>[2x]MNITKTLCLCAALSGAAGVQAMENREFVTQQDNTRVNNYQTNRPEAS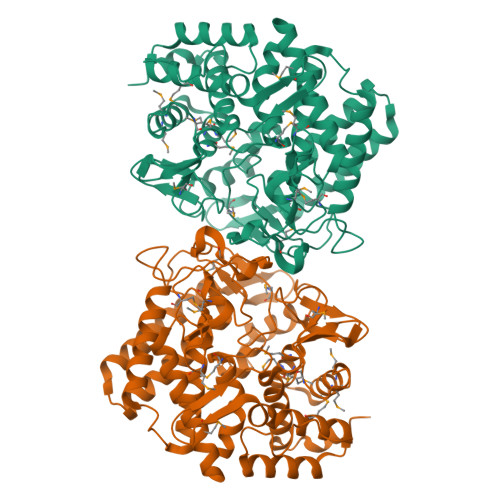KRLFVSQEVERQIDHIKQLLTNAKLAWMFENCFPNTLDTTVHFDGKEDTFVYTGDIHAMWLRDSGAQVWPYVQLANKDPELKKMLAGVINRQFKCINIDPYANAFNMNSEGGEWMSDLTDMKPELHERKWEIDSLCYPIRLAYHYWKTTGDASVFSDEWLQAIANVLKTFKEQQRKDDAKGPYRFQRKTERALDTMTNDGWGNPVKPVGLIASAFRPSDDATTFQFLVPSNFFAVTSLRKAAEILNTVNRKPALAKECTALADEVEKALKKYAVCNHPKYGKIYAFEVDGFGNQLLMDDANVPSLIALPYLGDVKVTDPIYQNTRKFVWSEDNPYFFKGSAGEGIGGPHIGYDMIWPMSIMMKAFTSQNDAEIKTCIKMLMDTDAGTGFMHESFNKNDPKNFTRAWFAWQNTLFGELILKLVNEGKVDLLNSIQLEHHHHHH> RASVGSPGIPAQDLPFVIKAGYLEKRRKDHSFLGFEWQKRWCALSKTVFYYYGSDKDKQQKGEFAIDGYDVRMNNTLRK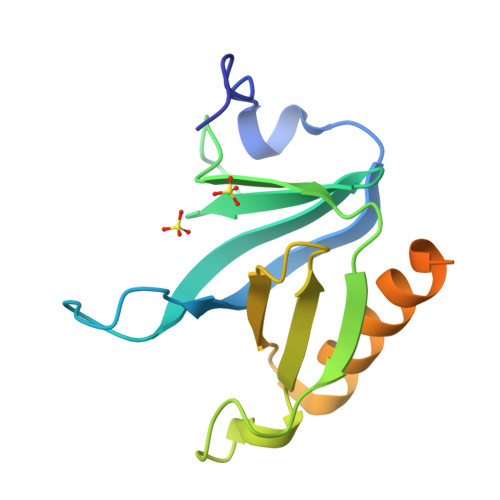DGKKDCCFEICAPDKRIYQFTAASPKDAEEWVQQLKFILQDLGSDVIPEDDEERGELYDDVDHPAAVSS> GAMGSRKSKAELQSEERKRIDEL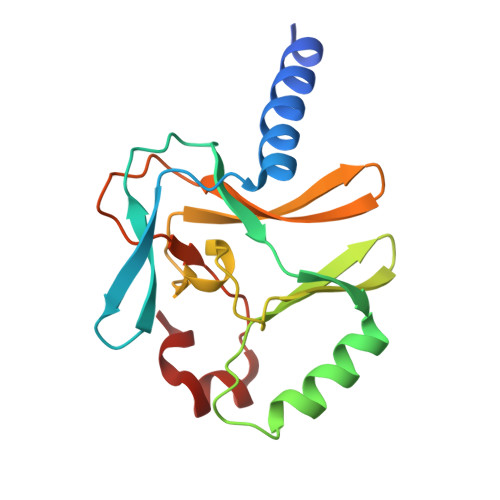IESGKEEGMKIDLIDGKGRGVIATKQFSRGDFVVEYHGDLIEITDAKKREALYAQDPSTGCYMYYFQYLSKTYCVDATRETNRLGRLINHSKCGNCQTKLHDIDGVPHLILIASRDIAAGEELLFDYGDRSKASIEAHPWLKH>[2x]MTIAVTGSIATDHLMRFPGRFSEQLLPEHLHKVSLSFLVDDLVMHRGGVAGNMAFAIGVLGGEVALVGAAGADFADYRDWLKARGVNCDHVLISETAHTARFTCTTDVDMAQIASFYPGAMSEARNIKLADVVSAIGKPELVIIGANDPEAMFLHT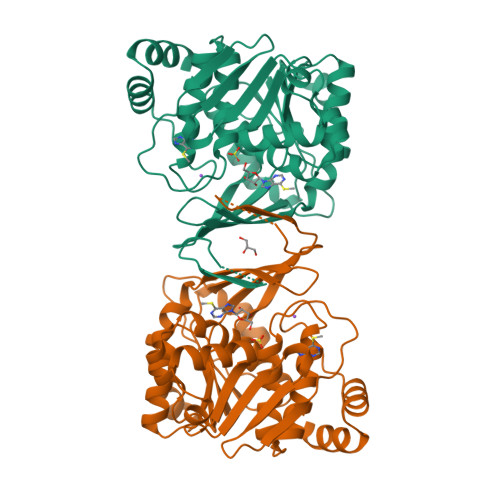EECRKLGLAFAADPSQQLARLSGEEIRRLVNGAAYLFTNDYEWDLLLSKTGWSEADVMAQIDLRVTTLGPKGVDLVEPDGTTIHVGVVPETSQTDPTGVGDAFRAGFLTGRSAGLGLERSAQLGSLVAVLVLESTGTQEWQWDYEAAASRLAGAYGEHAAAEIVAVLA> GAGCAGCCTGTACGGACATCAGATGCTGACGTAGTAGCAGAG;> CCGT;> TCCTCTGCTACTACGTCAGCATCTGATGT;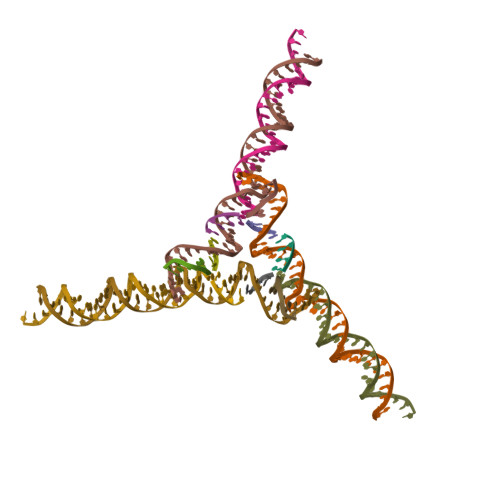> GGCTGC;> ACA> GMNAINTKVTPTKRKQVALFSSDPNFKRDVATRLDALAIYDVRVSETDDFLKGPPADTRPGI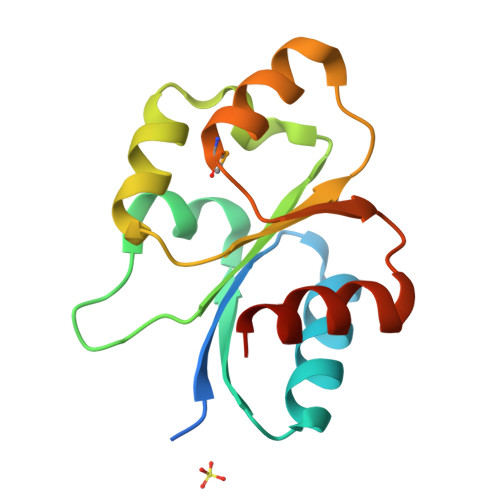VILDLGGGDLLGKPGIVEARALWATVPLIAVSDELTSEQTRVLVRMNASDWLHKPLDGKELLNAVTFHDTGNQ>PRVLVTGALGQIGTDLSLALRDKFGADSVLVSDVVEPGAKHPLAGLKGVEKLDCLDSNGFEKLVKEFKPTWMYHLPAIMSVRGEAEPDLAMDINVNTTRYALELARKYNIRIFIPSTIAAFGDKCGKTMTKDDTIMNPSTVYGVTKVYTELLGTWYRQKYGVDFRSVRLPGIISAATLPGGGATDYAIHMYHSALLQKKCVCPVLPYESLPMMYMPDTLNSLVKIMEAPLEKLTRTVYNITGFSFSPSELRFSIERCTDRTIEVEYVEGPAQKIANSWPDSLDDSNARNDWGHQVKYDIDMMSEDM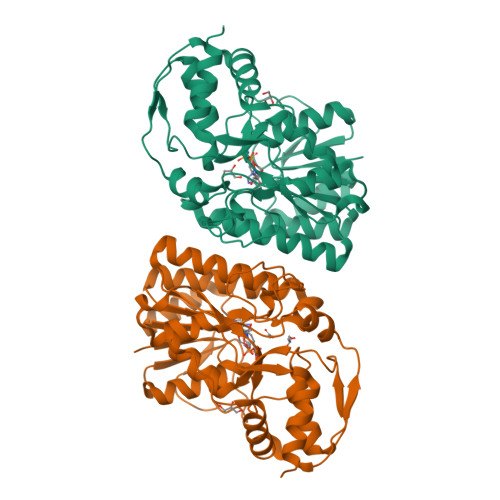LRQIPILHGLPSL[6x]[(~{Z})-[(3~{S},4~{R},5~{S},6~{S})-6-methyl-3,4,5-tris(oxidanyl)oxan-2-ylidene]amino] 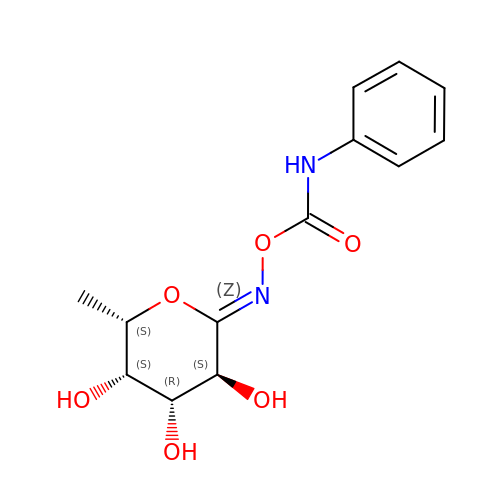~{N}-phenylcarbamate | C13 H16 N2 O6 | PUWMVMHIUFKDRR-SLDBRONRSA-N> MAGAGPTMLLREENGCCSRRQSSSSAGDSDGEREDSAAERARQQLEALL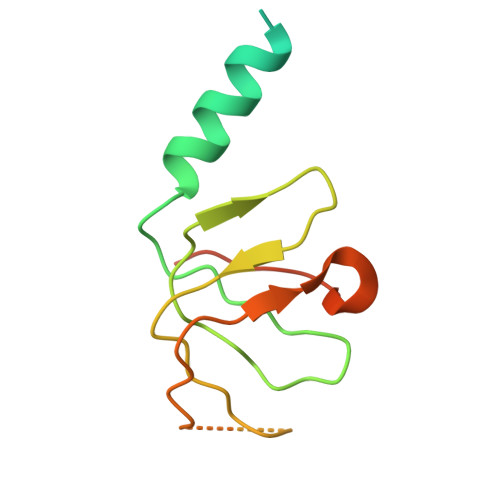NKTMRIRMTDGRTLVGCFLCTDRDCNVILGSAQEFLKPSDSFSAGEPRVLGLAMVPGHHIVSIEVQRESLTGPPYL>GPGSMTVEGFFDPATCTISYLLFDSGSGECALIDSVLDYDPKSGRTRTASADQLIARVAALGARVRWLLETHVHADHLSAAPYLKTRVGGEIAIGRHVTRVQDVFGKLFNAGPAFAHDGSQFDRLLDDGDTLALGALSIRAMHTPGHTPACMTYVVTEAHAAHDARDAAAFVGDTLFMPDYGTARCDFPGGDARSLYRSIRKVLSLPPATRLYMCHDYQPNGRAIQYASTVADELRENVHIREGVTEDDFVAMRTARDATLDMPVLMLPSV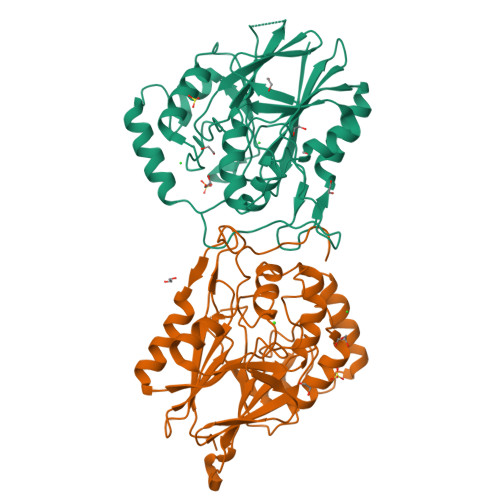QVNMRAGRLPEPEDNGVRYLKIPLDAI[2x]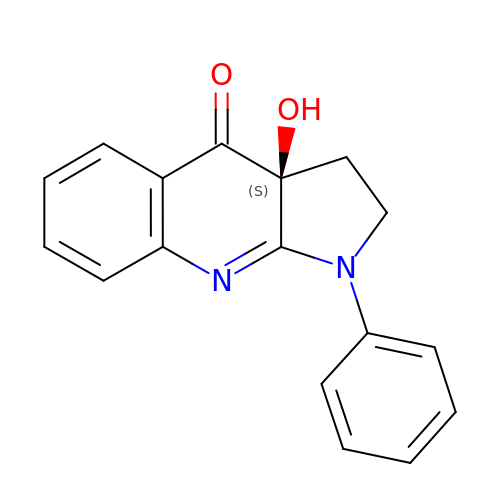(3aS)-3a-hydroxy-1-phenyl-1,2,3,3a-tetrahydro-4H-pyrrolo[2,3-b]quinolin-4-one | C17 H14 N2 O2 | DOMYOVZXZIZTRD-QGZVFWFLSA-N> MHSSGVARRQMRPYYNLPSKSEHGRRMTGFLTPYRHWMWKQNELWRNVHEAQFEHLRKLYKRQWLESFRVNADEYIYKYNITKSAQLAQWEHEMQGQERKRRESQQLAQGRQALKKKHLDLLREFHERQFFYWYERASERLQYMTHINYVPQASIQEHIDRELDKYTVGSKAPYPLNFVGQMPMLEDKDGNIAQVPANLMTNHATENPDGGVTMYEAPEGTAVAEEKLLQMIASAQEEELRIRPEDSDALSESMEDMDRSESARIDSRKVARTMEETDEEREVNRRAYIDRGKTGSKTIFRRPRLDSDGATPPSAGGTTPMKRRKSKMDRMHALQEQQDAVAAKATAKALKDEDSVAKATKRGEVAENRGRLRDRMIMPSLETLQQSPEM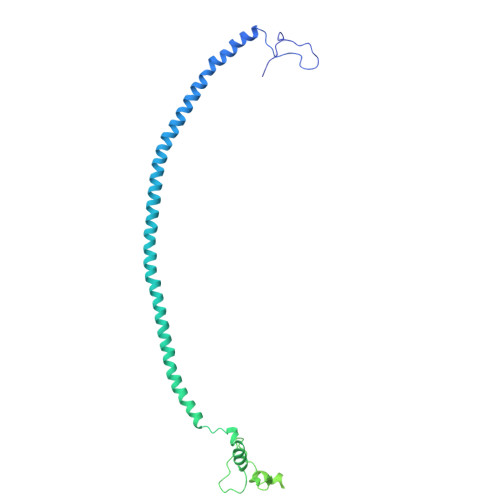MAQNKPGGRVRTHHLMEKVYGIGKFKKGGGGDEDA> MIPPRIVPWRDFAELEELKLWFYPKSKGTIEDKRQRAVQRVQSYRLKGSQYLPHVVDSTAQITCAVLLDEKEACLGVHQDSIPIRLSYVMALIRFVNGLLDPTQQSQFAIPLHTLAAKIGLPSWFVDLRHWGTHERDLPGLEMLRWAANEALSWLYDHYWNDEELEDDRDDDDDDDDTGYGYRRNDKLEKYMESLTKTLDKWKRLRNEFLEYKWVWENANDSLITSSNFSGDNLVNYDAEKRKSSHASSSETMIRENLRQWQELWKLSIYHNVVLEKFFNNYDPLLLKVLMLNLNNFDWKVIEWVARNYRTQQDDS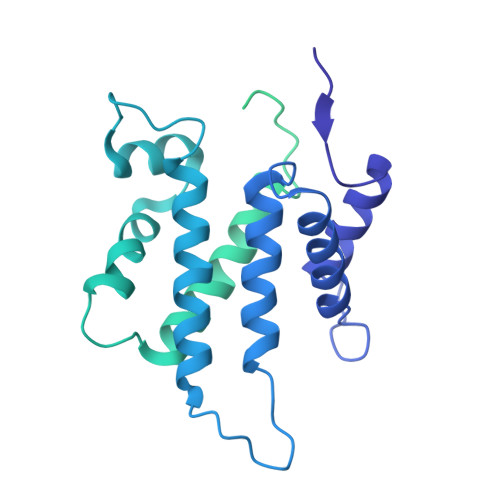NITTILKRKFNAWKELQKRLLDVIINNLNNKNFKNKWQNWEKLIDENASYLILYFCQSMLAKLETEKITGNSWRNKKRRKQIDSTVEIEAKLKENIDNLSLRFNEGEIKLYDFIPAEKDSVPLKKEVSPALKADTNDILGDLASLKQRMSSFGTVGKKNKQEENRATPVKNWSRVQNWKPKPFGVL> MILDKIVEDKKKRLEEHKAKIPPEEMKRMALECNRKTISLAKALSKPGLSIVAVFLKASPSKGVIRSKVDLEERIKQYNEAVDAITVVTEEDHFQGSPEYLKYIRERTNLPIIRWDFIIDEYQVYEAKVLGADAIFLIMAILDDETFKRLYDLAYSLGLDVVVLVYDEEELKRALNLGVKIIEIMNINLKTFEVSMDTTKRLASLLPEEFRKKDGILMTIGGISTDEDVKRLKKAGVDAF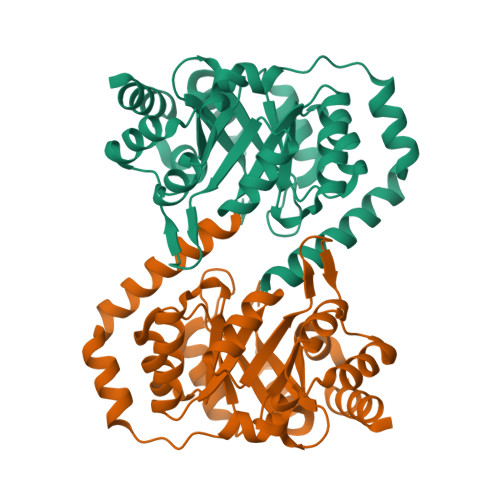VITEALMEADNPKELVKHWKEVYNNG> GPGSADASDWLNRLAEADRQNSFQGTFVYERNGSFSTHEIWHRVESDGAVRERLLQLDGARQEVVRVDGRTQCISGGLADQLADAQLWPVRKFDPSQLASWYDLRLVGESRVAGRPAVVLAVTPRDQHRYGFELHLDRDTGLPLKSLLLNEKGQLLERFQFTQLNTGAAPAEDQLQAGAECQVVGPAKADGEKTVAWRSEWLPPGFTLTR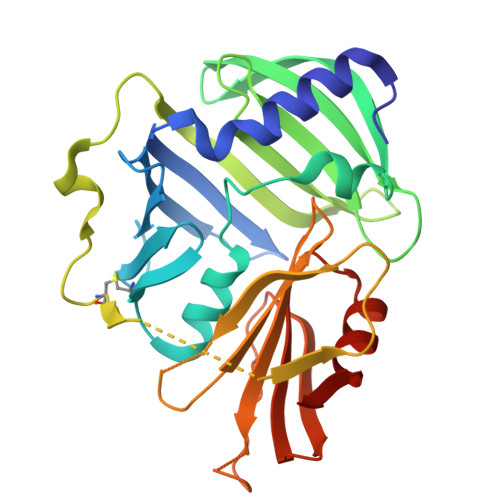SFMRRSPVTPDPVACLTYGDGLARFSVFIEPLHGAMVGDARSQLGPTVVVSKRLQTDDGGQMVTVVGEVPLGTAERVALSIRPEAAAQK>GHMKVDKLLVRLSDSVGYLFWDSATTGYATCFVFKGLFILTCRHVIDSIVGDGIEPSKWATI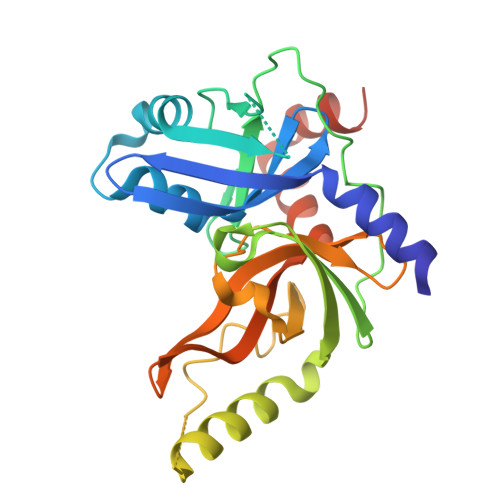IGQCVRVTFGYEELKDKETNYFFVEPWFEIHNEELDYAVLKLKENGQQVPMELYNGITPVPLSGLIHIIGHPYGEKKQIDACAVIPQGQRAKKCQERVQSKKAESPEYVHMYTQRSFQKIVHNPDVITYDTEFFFGASGSPVFDSKGSLVAMHAAGFAYTYQNETRSIIEFGSTMESILLDIKQRHKPWYEEVFVNQQDVEMMSDEDL[2x]[3-[(3~{R},4~{R})-3-(2-azanyl-6-oxidanylidene-1~{H}-purin-9-yl)-4-[(2~{S})-2-oxidanyl-2-phosphono-ethoxy]pyrrolidin-1-yl]-3-oxidanylidene-propyl]phosphonic 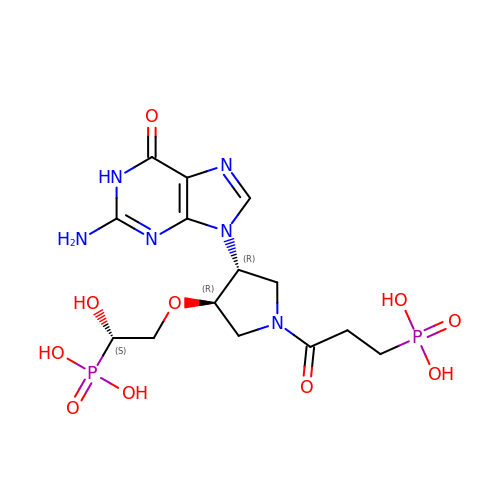acid | C14 H22 N6 O10 P2 | RBYFDIJTTUISNF-MRTMQBJTSA-N>MNITGKGAYDTGTYANLFQRSGYREDEIKARLEQTWNDLFYGDEHTRIYYPVGDDKGYMLDTGNDDVRSAGMSYGMMMAVQMDKKHEFDRLWNYAYTYMQHTEGRYKDYFAWHCKPDGTRLSPGPAPDGEEFFAMALFFASNRWGDGPAPYDYQAQARKILHACLHQGEQGEGDPMWEPSNRLIKFIPELPFSDPSYHLPHFYELFAQYANEQDRTFWKEAAEASRAYLRTACHPVTGLSPEYANYDGTPAPVQLHGDFRHFYSDAYRVAANVA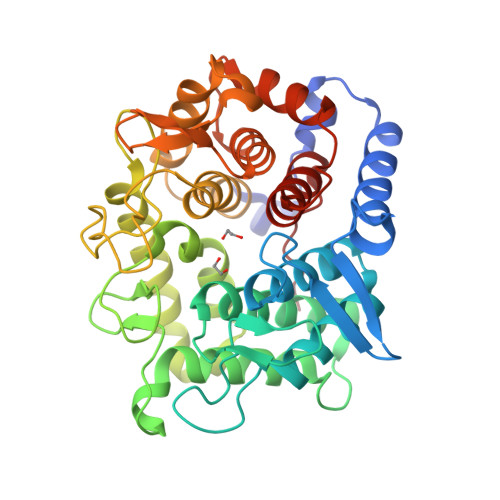LDWEWFRKDPWQVQQSNRIQAFFSDIDVSDYRRYTIEGEPFNEPALHPVGLLATNAMASLAADGPDADSFVKRFWNTPLRQGKRRYYDNCLYFFTMLALSGNYRVYQQ[2x]N-[(2S,3S,5R)-1-(3,5-difluorophenoxy)-3-hydroxy-5-(2-methoxyethoxy)-6-[[(2S)-3-methyl-1-oxo-1-(phenylmethylamino)butan-2-yl]amino]-6-oxo-hexan-2-yl]-5-(methyl-methylsulfonyl-amino)-N'-[(1R)-1-phenylethyl]benzene-1,3-dicarboxamide 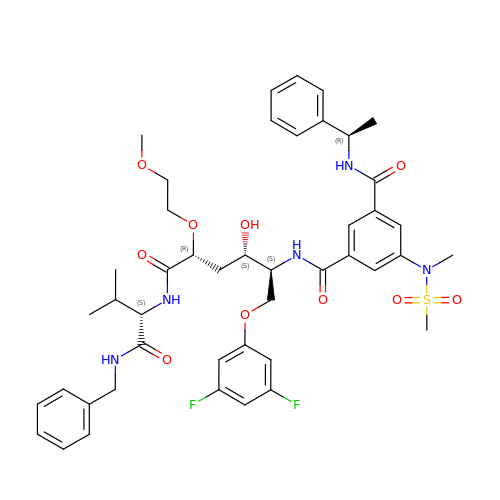| C45 H55 F2 N5 O10 S | RSTFVOGBJGGSOD-NDKACYJFSA-N>[4x]XVDAAVAKVCGSEAIKANLRRSWGVLSADIEATGLMLMSNLFTLRPDTKTYFTRLGDVQKGKANSKLRGHAITLTYALNNFVDSLDDPSRLKCVVEKFAVNHINRKISGDAFGAIVEPMKETLKARMGNYYSDDVAGAWAALVGVVQAAL;>[4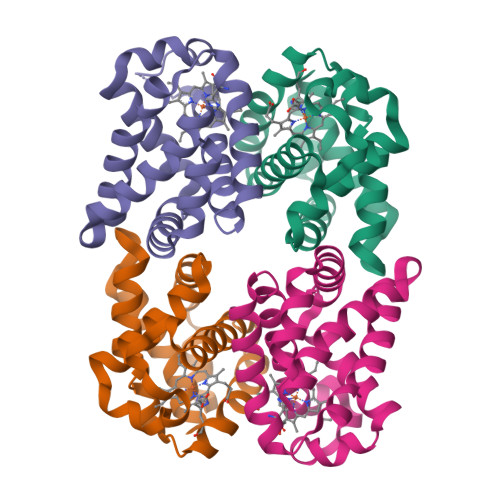x]XSRVAELANAVVSNADQKDLLRMSWGVLSVDMEGTGLMLMANLFKTSPSAKGKFARLGDVSAGKDNSKLRGHSITLMYALQNFVDALDDVERLKCVVEKFAVNHINRQISADEFGEIVGPLRQTLKARMGNYFDEDTVAAWASLVAVVQAAL>[2x]CC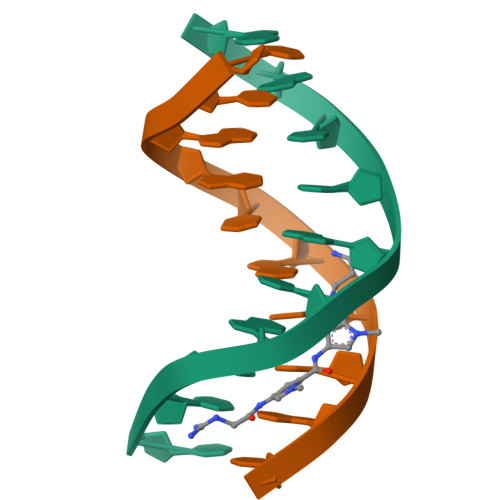IICICCII> QYSPNTQQGRTSIVHLFEWRWVDIALECERYLAPKGFGGVQVSPPNENVAIYNPFRPWWERYQPVSYKLCTRSGNEDEFRNMVTRCNNVGVRIYVDAVINHMCGNAVSAGTSSTCGSYFNPGSRDFPAVPYSGWDFNDGKCKTGSGDIENYNDATQVRDCRLTGLLDLALEKDYVRSKIAEYMNHLIDIGVAGFRLDASKHMWPGDIKAILDKLHNLNSNWFPAGSKPFIYQEVIDLGGEPIKSSDYFGNGRVTEFKYGAKLGTVIRKWNGEKMSYLKNWGEGWGFVPSDRALVFVDNHDNQRGHGAGGASILTFWDARLYKMAVGFMLAH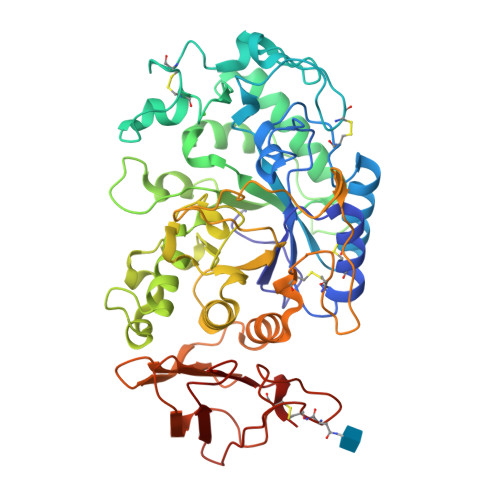PYGFTQVMSSYRWPRQFQNGNDVNDWVGPPNNNGVIKEVTINPDTTCGNDWVCEHRWRQIRNMVIFRNVVDGQPFTNWYDNGSNQVAFGRGNRGFIVFNNDDWSFSLTLQTGLPAGTYCDVISGDKINGNCTGIKIYVSDDGKAHFSISNSAEDPFIAIHAESKL>MAHHHHHHMVNVAVIGAAGGIGQSLSLLLLRELPFGSTLSLYDVVGAPGVAADLSHIDRAGITVKHAA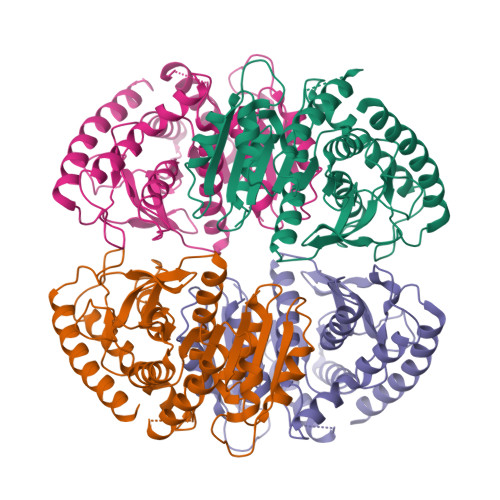GKLPPVPRDPALTELAEGVDVFVIVAGVPRKPGMTRDDLFNVNAGIVMDLVLTCASVSPNACFCIVTNPVNSTTPIAAQTLRKIGVYNKNKLLGVSLLDGLRATRFINNARHPLVVPYVPVVGGHSDVTIVPLYSQIPGPLPDESTLKEIRKRVQVAGTEVVKAKAGRGSATLSMAEAGARFTMHVVKALMGLDTPMVYAYVDTDGEHECPFLAMPVVLGKNGIERRLPIGPITTVEKEMLEEAVGVVKKNIAKGETFARSKL[4x]> HHHHHHGSAKKIVSDLDLKGKTVLVRADFNVPLKDGEITNDNRIVQALPTIQYIIEQGGKIVLFSHLGKVKEESDKAKLTLRPVAEDLSKKLDKE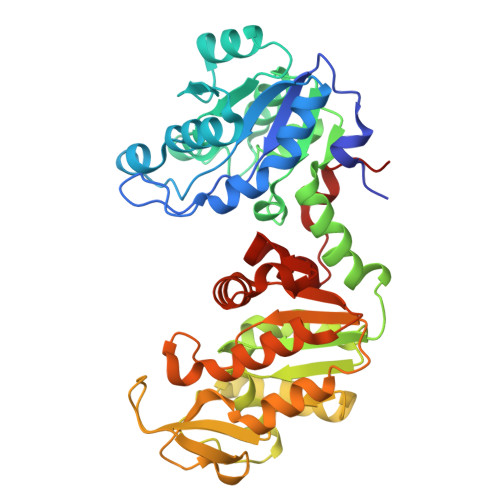VVFVPETRGEKLEAAIKDLKEGDVLLVENTRYEDLDGKKESKNDPELGKYWASLGDVFVNDAFGTAHREHASNVGISTHLETAAGFLMDKEIKFIGGVVNDPHKPVVAILGGAKVSDKINVIKNLVNIADKIIIGGGMAYTFLKAQGKEIGISLLEEDKIDFAKDLLEKHGDKIVLPVDTKVAKEFSNDAKITVVPSDSIPADQEGMDIGPNTVKLFADELEGAHTVVWNGPMGVFEFSNFAQGTIGVCKAIANLKDAITIIGGGDSAAAAISLGFENDFTHISTGGGASLEYLEGKELPGIKAINNK>[16x]XGGLEEIAQGLEEIAKGLKKIAWGLKKIAQGGX

Here we describe efficient routes starting from validated parallel and antiparallel peptide assemblies to design two families of α-helical barrel proteins with central channels that bind small molecules. Computational designs are seeded by the sequences and structures of defined de novo oligomeric barrel-forming peptides, and adjacent helices are connected by loop building. For targets with antiparallel helices, short loops are sufficient. However, targets with parallel helices require longer connectors; namely, an outer layer of helix–turn–helix–turn–helix motifs that are packed onto the barrels.

We solved high-resolution X-ray crystal structures of three peptides using ab initio phasing. Another structure, with g-a-d-e = Gly-Leu-Ile-Ala, had promising solution-phase data for an open hexamer or heptamer, but, interestingly, formed a collapsed antiparallel octamer in the crystal state. Some plasticity in assemblies formed from these types of peptides is expected. Thus, it is possible that Ala-Leu-Ile-Ala and Gly-Leu-Ile-Ala can also access an open conformation in solution.~{N}-[2,4-bis(fluoranyl)-3-[4-(3-methoxy-1~{H}-pyrazolo[3,4-b]pyridin-5-yl)-1,2,3-triazol-1-yl]phenyl]-3-bromanyl-benzenesulfonamide 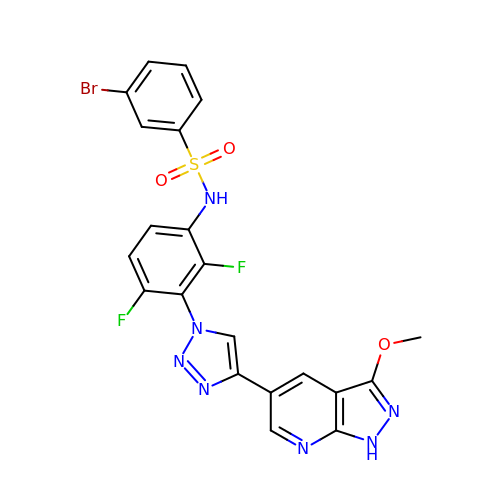| C21 H14 Br F2 N7 O3 S | XBRQXNKVCFFZSD-UHFFFAOYSA-N> GPLGSMASSNMKDETYYIALNMIQN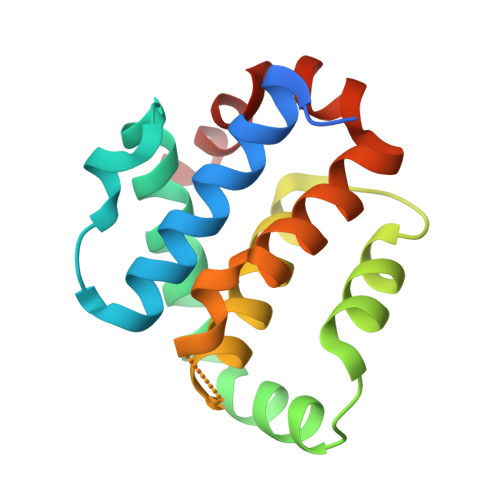YIIEYNTNKPRKSFVIDSISYDVLKAACKSVIKTNYNEFDIIISRNIDFNVIVTQVLEDKINWGRIITIIAFCAYYSKKVKQDTSPQYYDGIISEAITDAILSKYRSWFIDQDYWNGIRIYKN>[2x]SKSSSSRRNAWGNLSYADLITKAIESSAEKRLTLSQIYEWMVKSVPYFKDKGDSN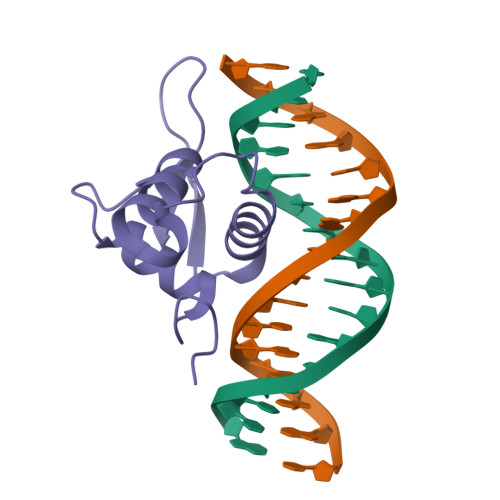SSAGWKNSIRHNLSLHSKFIRVQNEGTGKSSWWMLNPEGGKSGKSPRRRAASMDNNSKFAKS>NPSPHQVYNVTWTITNLVTGTKANATSMLGTLTDAFPTMYFDLCDIIGNTWNPSDQEPFPGYGCDQPMRRWQQRNTPFYVCPGHANRKQCGGPQDGFCAVWGCETTGETYWRPTSSWDYITVKKGVTQGIYQCSGGGWCGPCYDKAVHSSTTGASEGGRCNPLILQFTQKGRQTSWDGPKSWGLRLYRSGYDPIALFSV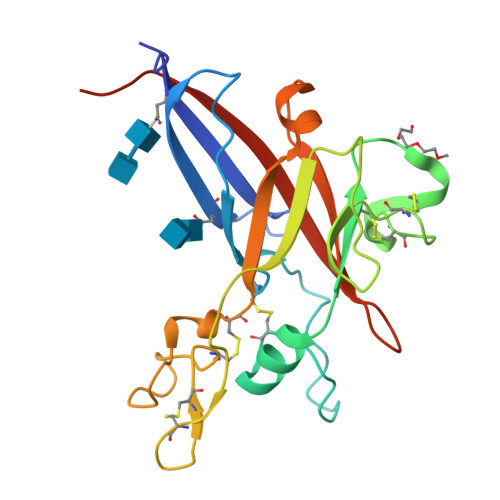SRQVMTITPPQA[2x]>[2x]AQPAVKHA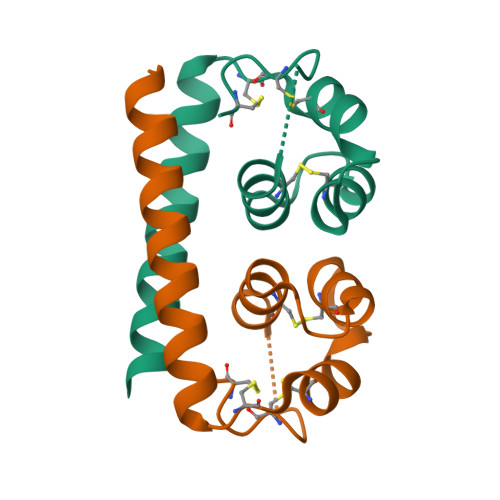LGQFNQVVTMFEKATAAASCNWITCLESLAASSAACAAALGELGLDIPLDLACIASAASTSAQGCEGCF> MIKKAVLPVAGLGTRFLPASKSIPKEMVTVVDRPAIEYVVREAVEAGIEQIILVTHSSKASIENYFDRNFELETTLEQKKKFDLLAEITQIVEEHVSVISVRQPQPLGLGHAVLCAKSVVGEDDFAVLLPDVLVKDGSGQNDLSRMISRYNSSQAAQIMVEAVPDHLVDQYGIVDVAQSPNEGESIAM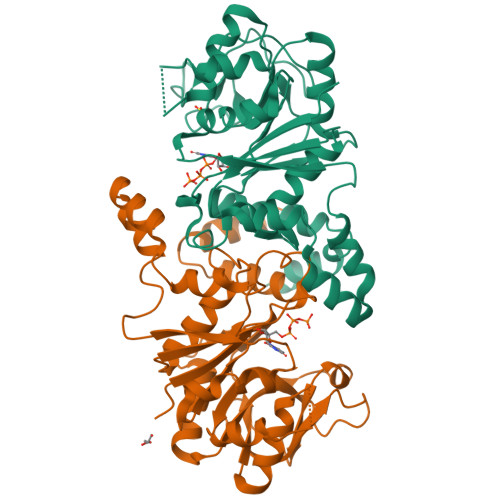QGIVEKPPVGAAPSNLSVVGRYVLPAKIMQLLENTPKGAGNEIQLTDAIAMLQDTDTVEAYRMQGQTFDCGSKLGYLKAVLHYGLEHPKLGMEFKQLILELK;> MIKKAVLPVAGLGTRFLPASKSIPKEMVTVVDRPAIEYVVREAVEAGIEQIILVTHSSKASIENYFDRNFELETTLEQKKKFDLLAEITQIVPEHVSVISVRQPQPLGLGHAVLCAKSVVGEDDFAVLLPDVLVKDGSGQNDLSRMISRYNSSQAAQIMVEAVPDHLVDQYGIVDVAQSPNEGESIAMQGIVEKPPVGAAPSNLSVVGRYVLPAKIMQLLENTPKGAGNEIQLTDAIAMLQDTDTVEAYRMQGQTFDCGSKLGYLKAVLHYGLEHPKLGMEFKQLILELK2-phenyl-N,N-dipropyl-1H-benzimidazole-5-sulfonamide | C19 H23 N3 O2 S 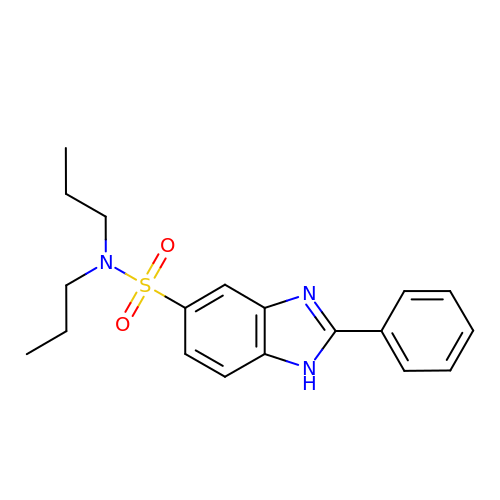| PFITZESRTBQCHT-UHFFFAOYSA-N>[2x]SGNFCPLCDKCYDDDDYESKMMQCGKCDRWVHSKCENLSDEMYEILSNLPESVAYTCVNCTERHPAEWRLALEKELQISLKQV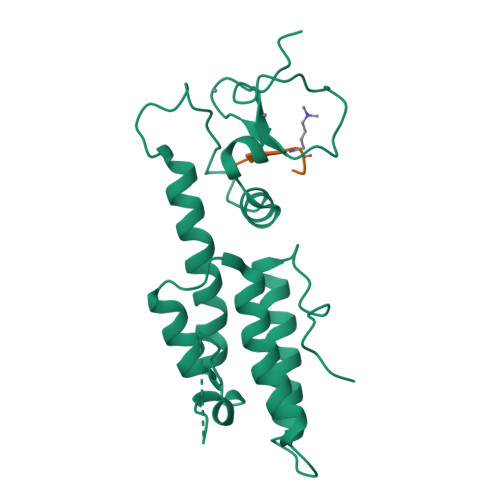LTALLNSRTTSHLLRYRQQQPLDLEGVKRKMDQGNYTSVLEFSDDIVKIIQAAINSDGGQPEIKKANSMVKSFFIRQMERVFPWFSVKKSRFWEPNKVSS;>ARTKQTARK[2x]>[8x]MLSPKAATLAERSAGLAFSLYQAMAKDQAVENILLSPVVVASSLGLVSLGGKATTASQAKAVLSAEQLRDEEVHAGLGELLRSLSNSTARNVTWKLGSRLYGPSSVSFAEDFVRSSKQHY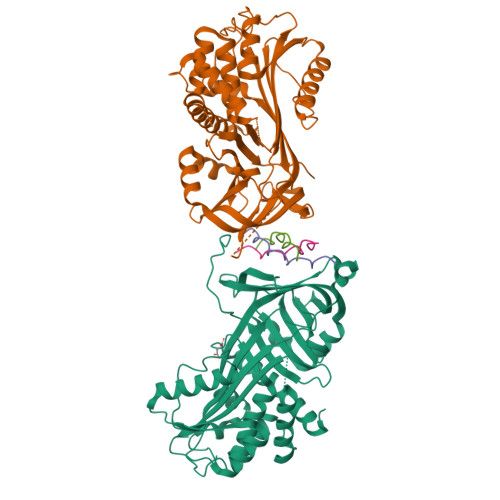NCEHSKINFRDKRSALQSINEWAAQTTDGKLPEVTKDVERTDGALLVNAMFFKPHWDEKFHHKMVDNRGFMVTRSYTVGVTMMHRTGLYNYYDDEKEKLQIVEMPLAHKLSSLIILMPHHVEPLERLEKLLTKEQLKIWMGKMQKKAVAISLPKGVVEVTHDLQKHLAGLGLTEAIDKNKADLSRMSGKKDLYLASVFHATAFEWDTEGNPFDQDIYGREELRSPKLFYADHPFIFLVRDTQSGSLLFIGRLVRPKGDKMRDELLEHHHHHH;>[12x]XPPGPPGPTGPRGPPGPPX[(2R)-7-(2-aminopyridin-4-yl)-5-chloro-2,3-dihydro-1-benzofuran-2-yl](piperazin-1-yl)methanone | C18 H19 Cl N4 O2 | 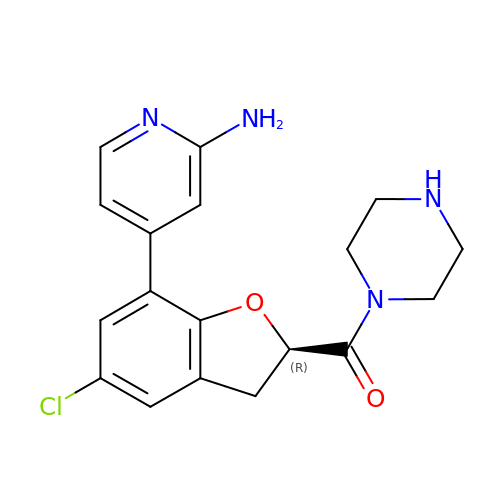JGHCITCCEQEXTL-OAHLLOKOSA-N>[4x]LVSSPSTLNPGTNVAKLAEQAPVHWVSVAQIENSLTGRPPMAVGFDIDDTVLFSSPGFWRGKKTYSPDSDDYLKNPAFWEKMNNGWDEFSIPKEAARQLIDMHVRRG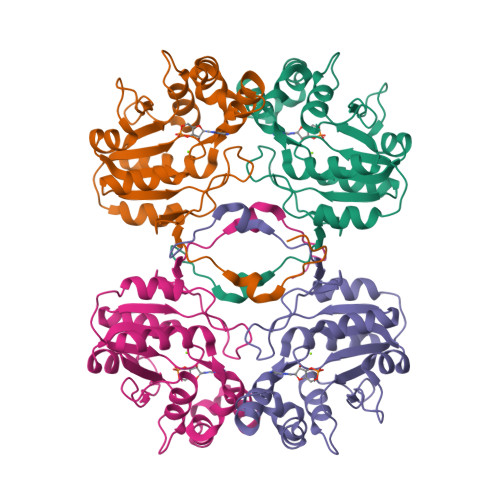DSIYFVTGRSQTKTETVSKTLADNFHIPAANMNPVIFAGDKPEQNTKVQWLQEKNMRIFYGDSDNDITAARDCGIRGIRILRAANSTYKPLPQAGAFGEEVIVNSEY>GSNNVPKNASALLRMNFVKGNQVLSGTGSATFIAPNVLLTVAHNFINNSADNSTGEFIGDKSKNTYEWQTPDGQKGSFTSEDIHFYNKKDYPKGFIYDLAVITLPQSTRRQHANLVENYSKVNVNDKLNVYGYPRGEYAHLKDTTVEIEQKYANNTYGVQYQGGKAGMSGGGIFNSKGEVIGLHQNGAENRSGGLILSPTQLDWIRSIIKGKEIT[2x]

Immunoglobulin A proteases (IgAPs) represent an interesting group of proteolytic enzymes that have convergently evolved to specifically cleave the unique hinge region present in IgA1 from humans and great apes via several different chemical mechanisms. The M26 IgAP family can be split into two subfamilies with distinct domain architectures. The subfamily represented by the Gemella haemolysans IgAP (GhIgAP) contains an additional trypsin-like domain (GhTrp) found N-terminal to the IgAP domain (residues 684–8961; Redzic et al., 2022). Prior studies that compared GhIgAP constructs with and without this domain concluded that GhTrp had no effect on IgA1 proteolysis.

The 1.75 Å resolution structure of the G. haemolysans M26 IgA1 protease trypsin-like domain is presented. To gain insight into the structure and potential functional role of this domain, we solved the crystal structure of GhTrp and demonstrated that the domain does indeed possess a trypsin-like protease fold. This fold, however, contains many unique changes in the well characterized surface loops that are known to contribute to trypsin-like protease specificity. As expected, the GhTrp crystal structure depicts two molecules in the asymmetric unit, related to each other along the c axis by a tNCS vector of approximately half the c-axis length. Despite having low sequence identity (<20%) to most known chymotrypsin-like and trypsin-like proteases, DALI analysis demonstrates that the fold of GhTrp is consistent with other members of the S1 family of glutamyl endopeptidases, as categorized by the MEROPS database. Loop 1, which contains the serine nucleophile (Ser167) and the oxyanion-hole residues (amides of Ser167/Gly165), is similar in structure between GhTrp and BGP but is truncated when compared with bovine trypsin. Taken together, these data suggest that the GhTrp structure could represent a pro-enzyme-like form of the putative zymogen in which some activation event is required to properly stabilize loop 2 in an active conformation to generate a viable S1 pocket. We hypothesize that this putative pro-enzyme form must undergo a specific cleavage event to generate an N-terminal segment that interacts with loop 2 to stabilize a more open and active conformation of the S1 pocket.>MKHHHHHHHHGGLVPRGSHGMTKKIVAIWAQDEEGVIGKDNRLPWYLPAELQHFKETTLNHAILMGRVTFDGMGRRLLPKRETLILTRNPEEKIDGVATFHDVQSVLDWYSAQEKNLYIVGGKQIFQAFEPYLDEVIVTHIHARVEGDTYFPAEFDLSLFETVSSKFYTKDEKNPYDFTIQYRKRKE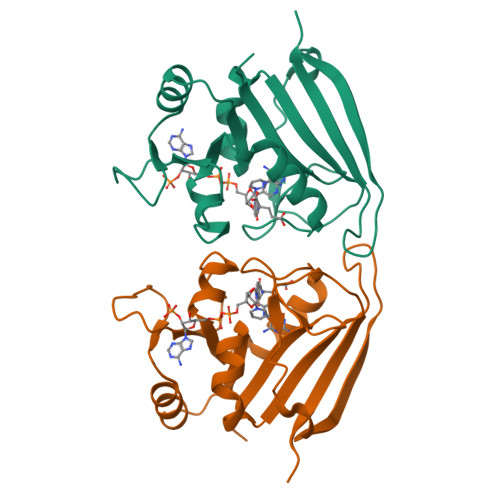VLE[2x]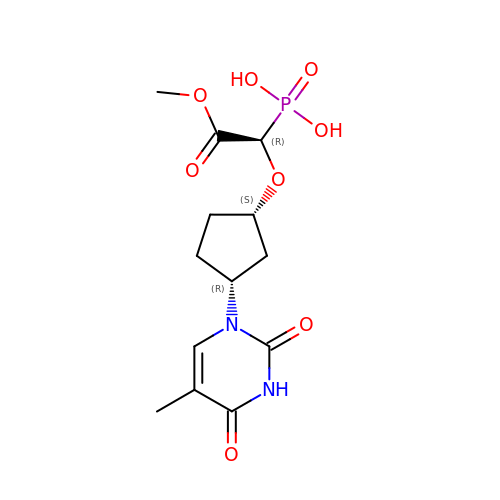[(1R)-2-methoxy-1-{[(1S,3R)-3-(5-methyl-2,4-dioxo-3,4-dihydropyrimidin-1(2H)-yl)cyclopentyl]oxy}-2-oxoethyl]phosphonic acid | C13 H19 N2 O8 P | VZWKSNLNIFIGPO-VDDIYKPWSA-N PYRIMIDINE-2,4,6-TRIAMINE | C4 H7 N5 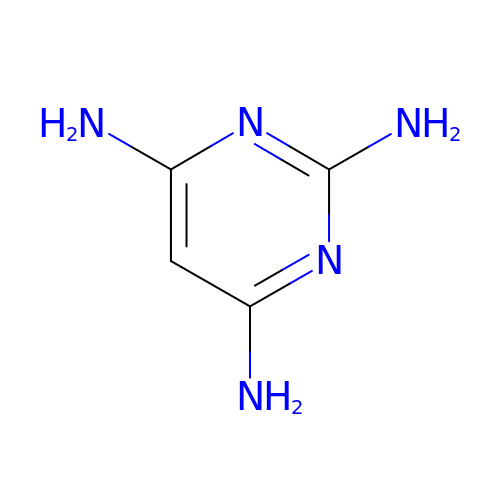| JTTIOYHBNXDJOD-UHFFFAOYSA-N>GMARLKNLPQERPLPLASLIEARENQVLSMALAQSDRVQISLFSFADGESVSEEEYFGDTLYLILQGEAVITFDDQKIDLVPEDVLMVPAHKIHAIAGKGRFKML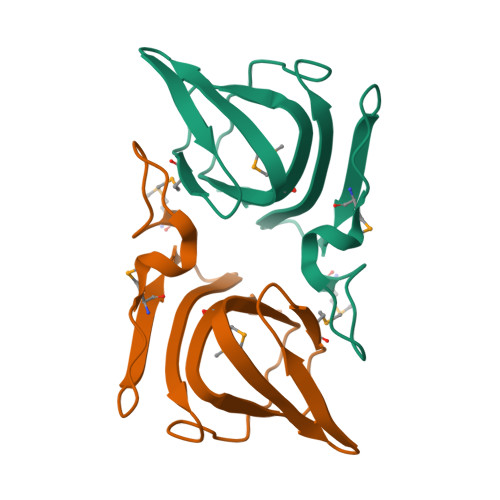QITLIDEER[2x]> MAHHHHHHALEVLFQGPISPIETVPVKLKPGMDGPKVKQWPLTEEKIKALVEICTEMEKEGKISKIGPENPYNTPVFAIKKKDSTKWRKLVDFRELNKRTQDFWEVQLGIPHPAGLKKKKSVTVLDVGDAYFSVPLDEDFRKYTAFTIPSINNETPGIRYQYNVLPQGWKGSPAIFQSSMTKILEPFKKQNPDIVIYQYMDDLYVGSDLEIGQHRTKIEELRQHLLRWGLTTPDKKHQKEPPFLWMGYELH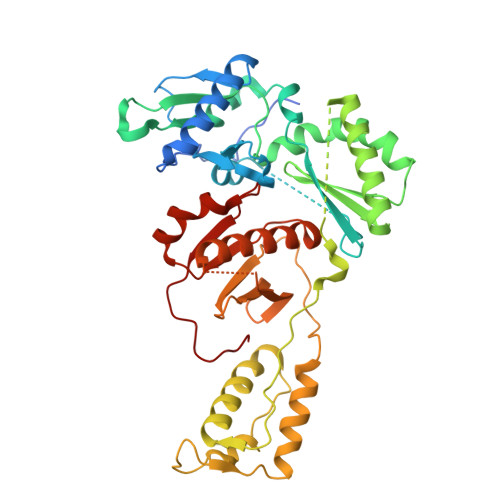PDKWTVQPIVLPEKDSWTVNDIQKLVGKLNWASQIYPGIKVRQLCKLLRGTKALTEVIPLTEEAELELAENREILKEPVHGVYYDPSKDLIAEIQKQGQGQWTYQIYQEPFKNLKTGKYARMRGAHTNDVKQLTEAVQKITTESIVIWGKTPKFKLPIQKETWETWWTEYWQATWIPEWEFVNTPPLVKLWYQ S-layer proteins (SLPs) are self-assembling, crystalline proteins coating the cell surfaces of many prokaryotes. We determined the atomic resolution structures of all functional domains (I-III from N- to C-termini) present in the three S-layer proteins SlpA_ac, SlpX_ac, and SlpA_amy. The Lactobacillus S-layers are anchored to the cell wall through interaction with teichoic acids (TA), either lipoteichoic acid (LTA) or wall teichoic acid (WTA).

The full-length SlpX_ac shows differences in structure and domain arrangement compared to the SlpA architecture. The middle domain of SlpX, SlpX_ac_II, exhibits a SlpA_I-like domain fold and an additional repeat of the SlpA motif. The four residues observed in the vicinity of phosphates are conserved with the proposed binding motif of YxY….KxxN. These residues are not conserved in the third SlpA-motif, which is present in SlpX_ac_II. However, SlpX_ac_II contains an additional 3rd SlpA motif and an additional loop region, allowing for increased protein flexibility to incorporate into the assembled SlpA-SlpX S-layer.

>[4x]MGSTPTDTTQNPQINWTKGGQAQSSSLNGQVFQVAVGSNFNPLNFTNSNGENIIVSAQQSKNNTTFASIEATSNPVNTSEAGRYYNVTLTATGNTGKKTTATYTVLITSSQKQTLYGNGESTISTYSIYGNNVLCNSTTFKDGDQVYVSDQTKTVGGVSYSQVSPKSKNDANSSNIWVKTSLEHHHHHH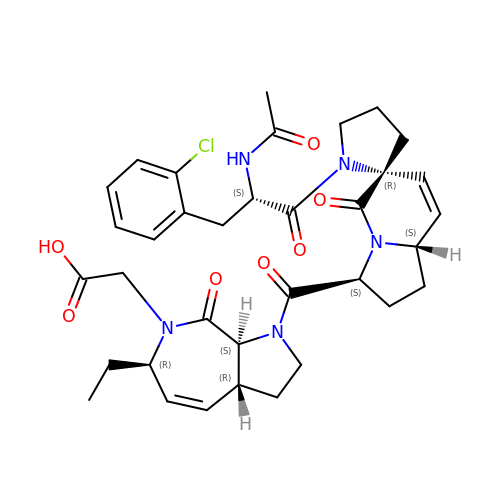2-[(3~{a}~{R},6~{R},8~{a}~{S})-1-[(3~{S},6~{R},8~{a}~{S})-1'-[(2~{S})-2-acetamido-3-(2-chlorophenyl)propanoyl]-5-oxidanylidene-spiro[1,2,3,8~{a}-tetrahydroindolizine-6,2'-pyrrolidine]-3-yl]carbonyl-6-ethyl-8-oxidanylidene-3,3~{a},6,8~{a}-tetrahydro-2~{H}-pyrrolo[2,3-c]azepin-7-yl]ethanoic acid | C35 H42 Cl N5 O7 | VKBPCLAGXRQASF-TUFUIHJKSA-N>GMTEIQTIRKKVEQQITSLQNETDEIAEFNQAKVLDAFQENKVSDFHFNPSTGYGYDDEGRDTLERVYASVFKTEAALVRPQIISGTHAISTVLFGILRPGDELLYITGEPYDTLEEIVGIRSEGQGSLKDFQIGYDAVPLLPNGEIDYPAVSKKISANTKMIGIQRSRGYADRPSFTIEKIKEMVTFVKNINPNIIVFVDNCYGEFVERIEPTEVGADIIAGSLIKNPGGGLAKTGGYIAGRNTLVDLCGYRLTTPGIGREAGASLYSLLEMYQGFFLAPHVTAQAIKGARFTAAMLAEFGVEADPLWDAKRTDLIQSVSFHSKDKMIAFAQAIQAASPVNAHVLPIGA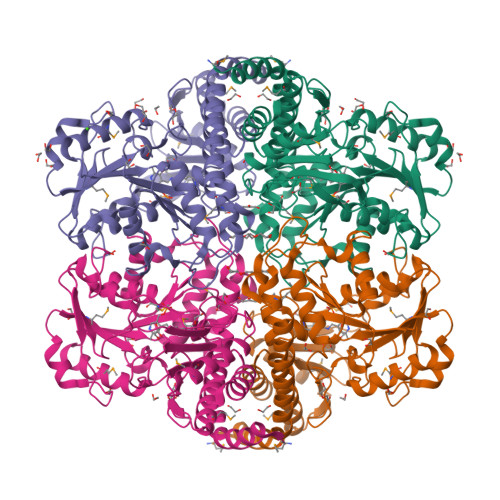YMPGYEDDVIMAAGTFIQGASLELTADGPIREPYQLYVQGGLTYEHVKIAVTRAIENSL[2x]>MTDTDSPAPAPSPSRRSLIGWGGAGLALGAAAAAGGAVAMDRAGADADPAGADAGSAVPFHGAHQAGIATPVQDRLHFAAFDVTTEDRAAFVALLKEWTAAARRLTAGHAVGEGAYGGLPEAPPDDTGEALGLKPSRLTLTIGFGPSLFTRFGLADLRPEALADLPKFPGDNLDRARSGGDLCVQACADDPQVAVHAIRNLARIGFGKVVVRWSQLGFGKTSSTTPDKQTPRNLLGFKDGTRNIAGTEKDRLDRFVWAAEKDGTPWMTGGSYLVARRIRMHIETWDRASLQEQEDVFGRDKGEGAPVGKAKERDEPFLKAMKPDAHVRLAHPDSNGGATLLRRGFSYTDGTDGLGRLDAGLFFLAYQRDIRTGFVPVQRNLATDALNEFIQHVGSAVFAVPPGVRDADDWWGSTLFG[2x]

Dye-decolourising peroxidases (DyPs) are a distinct structural family of peroxidases possessing an α + β dimeric fold that houses a b-type heme coordinated on its proximal side by a His residue. The soil dwelling bacterium, Streptomyces lividans possesses three DyPs; two belonging to the A-type and a third belonging to the B-type sub-families. The two A-type homologs, named DtpA and DtpAa react in their ferric heme state with H2O2 to form a two-electron oxidised derivative that is an Fe(iv)O heme carrying a porphyrin π-cation radical (Fe(iv)O[Por˙+]) – termed compound I.34–36 In the presence of a substrate, reduction of the porphyrin π-cation radical results in the formation of compound II (Fe(iv)O), with a second substrate molecule reducing compound II to the ferric state. By using an A-type member of the DyP family (DtpAa) as an exemplar, we combine protein engineering, X-ray crystallography, hole-hopping calculations, EPR spectroscopy and kinetic modelling to provide compelling new insights into the control of radical migration pathways following reaction of the heme with hydrogen peroxide.

The triple variant, Y345F/F347Y/Y389F, now mimics the Tyr arrangement on the distal heme side and the proximal Trp environment of DtpA. The X-ray crystal structure of the triple variant was determined to 1.50 Å resolution, confirming the presence of the introduced proximal Phe, and further corroborated the integrity of the structural H2O in proximity of Tyr347 and Asp358. Finally, disrupting the charge distribution of the Trp285/Tyr389 dyad in the triple variant, results in only two calculated routes, one to the proximal Trp and the second to the engineered distal Tyr347. By contrast to this low intensity free radical signal in the double variant, the triple variant (mimics DtpA on both distal and proximal heme) gave a strong EPR signal in the g = 2 region (compared to the double variant) with a line shape and microwave power saturation behaviour consistent with being caused by an uncoupled (not coupled to heme iron) protein radical. Spectral simulation of the radical signal was successfully achieved using TRSSA-Y.v2,35 unambiguously confirming it to be caused by a YO˙ species. Therefore, based on the near identical line shapes of the YO˙ species in the triple variant of DtpAa, and WT DtpA,35 we assign the YO˙ species in the triple variant to the engineered Tyr347 – the position homologous to 374 in DtpA. However, in the triple variant in which charge distribution over the ETA components of the dyad (Trp285/Tyr389) is disrupted by replacing the Tyr with a Phe, SigB is lowly populated and the YO˙ species (Tyr347) is almost fully populated.> MLNYNAPTDGQKSSIDGANSDQMQTFFWLKKAIITARKEQYFMPLASVTNMPKHYGKTIKVYEYVPLLDDRNINDQGIDASGATIVNGNLYGSSKDIGNITSKLPLLTENGGRVNRVGFTRIAREGSIHKFGFFYEFTQESIDFDSDDGLMEHLSRELMNGATQITEAVLQKDLLAAAGTVLYAGAATSDATITGEGSTPSVVSYKNLMRLDQILTENRTPTQTTIITGSRMIDTKVIGATRVMYVGSELVPELKAMKDLFGNKAFIETQHYADAGTIMNGEVGSIDKFRIIQVPEMLHWAGAGAQATGANPGYRTSMVSGQEHYDVYPMLVVGDDSFTSIGFQTDGKSLKFTVMTKMPGKETADRNDPYGETGFSSIKWYYGILVKRPERL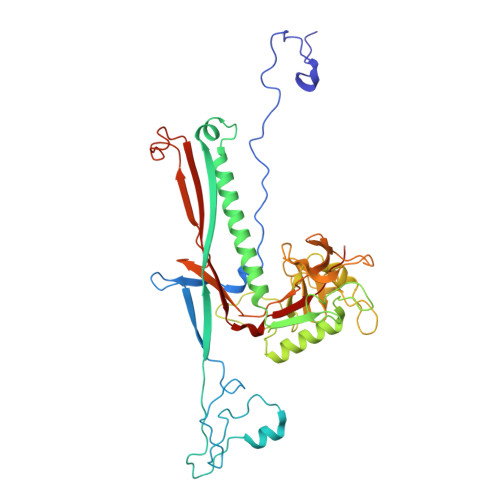ALIKTVAPL>MGSSHHHHHHSSGLVPRGSRVLSIQSHVIRGYVGNRAATFPLQVLGFEIDAVNSVQFSNHTGYAHWKGQVLNSDELQELYEGLRLNNMNKYDYVLTGYTRDKSFLAMVVDIVQELKQQNPRLVYVCDPVLGDKWDGEGSMYVPEDLLPVYKEKVVPLADIITPNQFEAELLSGRKIHSQEEALRVMDMLHSMGPDTVVITSSDLPSPQGSNYLIVLGSQRRRNPAGSVVMERIRMDIRK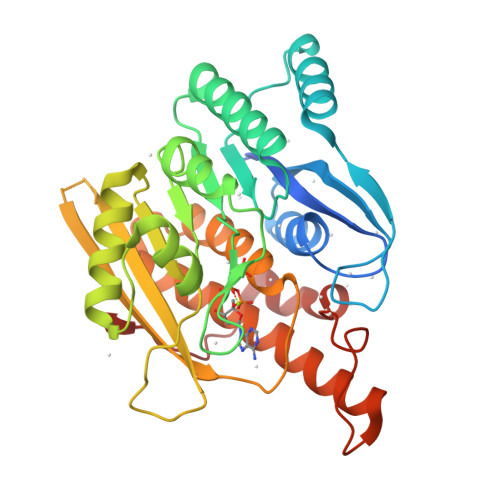VDAVFVGTGDLFAAMLLAWTHKHPNNLKVACEKTVSTLHHVLQRTIQCAKAQAGEGVRPSPMQLELRMVQSKRDIEDPEIVVQATVL[2x]4-{[2-(4-{[(4-FLUOROPHENYL)CARBONYL]AMINO}-1H-PYRAZOL-3-YL)-1H-BENZIMIDAZOL-6-YL]METHYL}MORPHOLIN-4-IUM 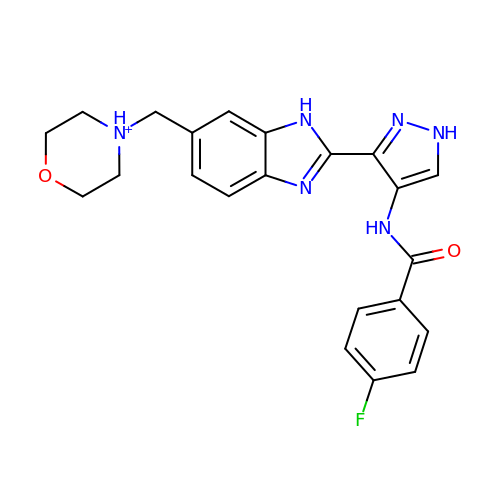| C22 H22 F N6 O2 | AKIIIZOJWRPEPQ-UHFFFAOYSA-O> MAGNSGSGAAAAAN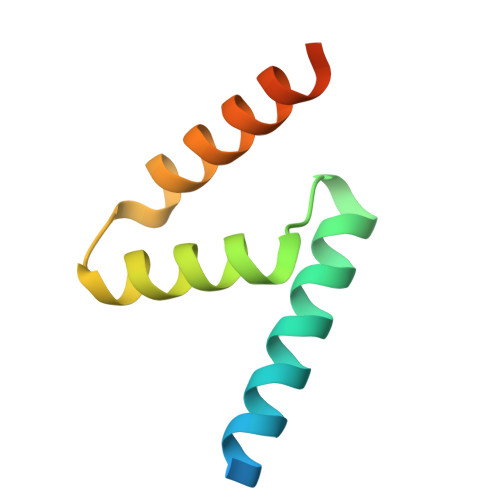LNAVRETMDVLLEISRILNTGLDMETLSICVRLCEQGINPEALSSVIKELRKATEALKAAENMTS> ELTQSRVQKIWVPVNSPTVIVMVGLPARGKTYISKKLTRYLNWIGVPTKVFNVGEYRREAVKQYSSYNFFRPDNEEAMKVRKQCALAALRDVKSYLAKEGGQIAVFDATNTTRERRHMILHFAKENDFKA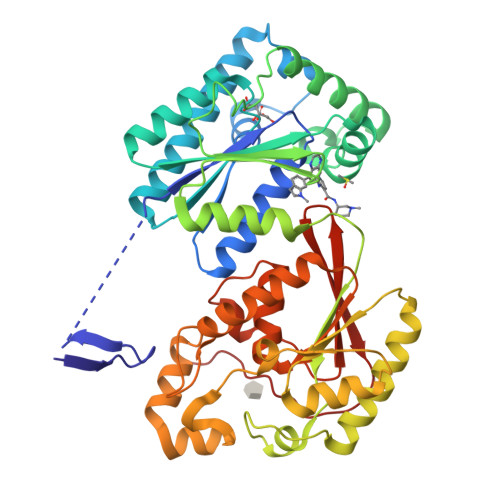FFIESVCDDPTVVASNIMEVKISSPDYKDCNSAEAMDDFMKRISCYEASYQPLDPDKCDRDLSLIKVIDVGRRFLVNRVQDHIQSRIVYYLMNIHVQPRTIYLCRHGENEHNLQGRIGGDSGLSSRGKKFASALSKFVEEQNLKDLRVWTSQLKSTIQTAEALRLPYEQWKALNEIDAGVCEELTYEEIRDTYPEEYALREQDKYYYRYPTGESYQDLVQRLEPVIMELERQENVLVICHQAVLRCLLAYFLDKSAEEMPYLKCPLHTVLKLTPVAYGCRVESIYLNVESVCTHRERSE> GDRVADVIESSIGDSVSRALTHALPAPTGQNTQVSSHRLDTGKVPALQAAEIGASSNASDESMIETRCVLNSHSTAET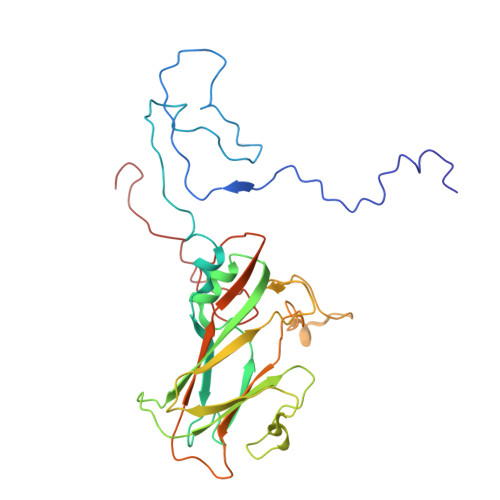TLDSFFSRAGLVGEIDLPLKGTTNPNGYANWDIDITGYAQMRRKVELFTYMRFDAEFTFVACTPTGEVVPQLLQYMFVPPGAPKPDSRESLAWQTATNPSVFVKLSDPPAQVSVPFMSPASAYQWFYDGYPTFGEHKQEKDLEYGAMPNNMMGTFSVRTVGTSKSKYPLVVRIYMRMKHVRAWIPRPMRNQNYLFKANPNYAGNSIKPTGASRTAITTL> SMAAQKNNAPKEYGADSITILEGLEAVRKRPGMYIGSTGERGLHHLIWEVVDNAVDEAMAGFATRVDVKIHADGSVEVRDDGRGIP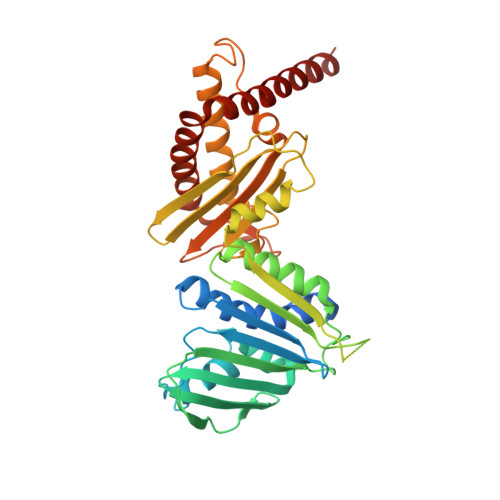VEMHATGMPTIDVVMTQLHAGGKFDGETYAVSGGLHGVGVSVVNALSTRLEATVLRDGYEWFQYYDRSVPGKLKQGGETKETGTTIRFWADPEIFETTDYNFETVARRLQEMAFLNKGLTIELTDERVTAEEVVDDVVKDTAEAPKTADEKAAEATGPSKVKHRVFHYPGGLVDYVKHINRTKTPIQQSIIDFDGKGPGHEVEIAMQWNAGYSESVHTFANTINTHEGGTHEEGFRAALTSVVNRYAKDKKLLKDKDPNLTGDDIREGLAAVISVKVAEPQFEGQTKTKLGNTEVKSFVQKICNEQLQHWFEANPAEAKTVVNKAVSSAQARIAARKARELV> MLVPGLSLTRRAVTSSCCRPLHVVRGFSTTCTLFGLEQLQDVPTSTSRRPTGLHRGPGKRQTSEREAAQYKFIRRWELQMRDEWDQLEPFKGLPKPKRQFGNEAAEVIWPYALLLERVVKVHPFTKSIYVYYAQRQSTARGKLAAEIAR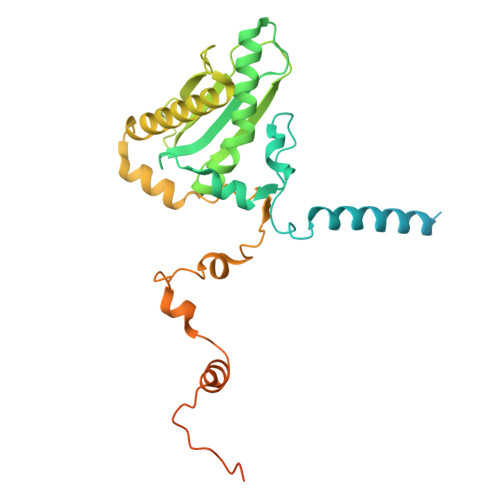SFAREFLIPITFHNSQVYTEAEMLLEYSETPWVVLHSLDNGQKPRILPVAPVEGTPAHTAVEQLLAEVVQGCEALGASVADPVTATRVLNERPLQNQYVRVDYQWFGDTPDERASHLVRWEFEPEQIEPKIRHRTRHVLDWLNYDGNLPTHRAVHVNAMREKARQKAPRTVAGPRTFYNSAGSRANARSSRFGGQAAVGK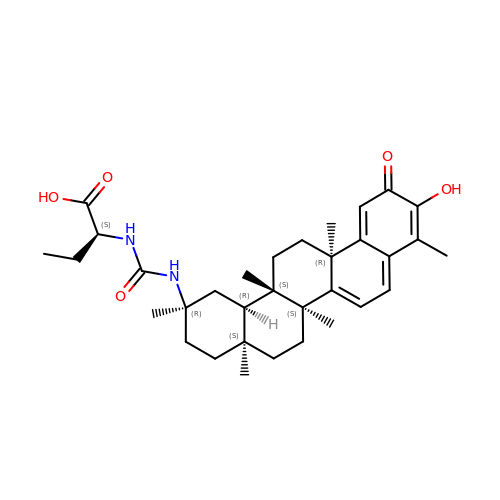(2~{S})-2-[[(2~{R},4~{a}~{S},6~{a}~{R},6~{a}~{S},14~{a}~{S},14~{b}~{R})-2,4~{a},6~{a},6~{a},9,14~{a}-hexamethyl-10-oxidanyl-11-oxidanylidene-1,3,4,5,6,13,14,14~{b}-octahydropicen-2-yl]carbamoylamino]butanoic acid | C33 H46 N2 O5 | PMMICXSXMUCBMJ-XSZYYSLISA-N>[2x]MGSDKIHHHHH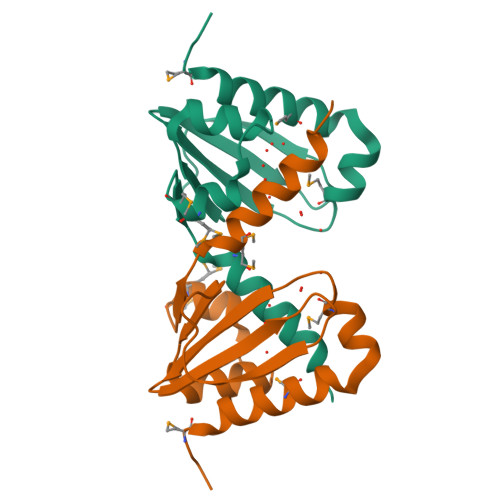HMSEAKELIKKMCDLQNSNEEIQKEMAGWSGVVQYKLDGYYFYVEYKSDGTCEFKEGVHSSPTFTVVAPPDFWLAVLKGQEDPVSGFMMGKYRIEGNIMEAQRLAGVIKKFQGKFEL>MGKVYKKVELVGTSEEGLEAAIQAALARARKTLRHLDWFEVKE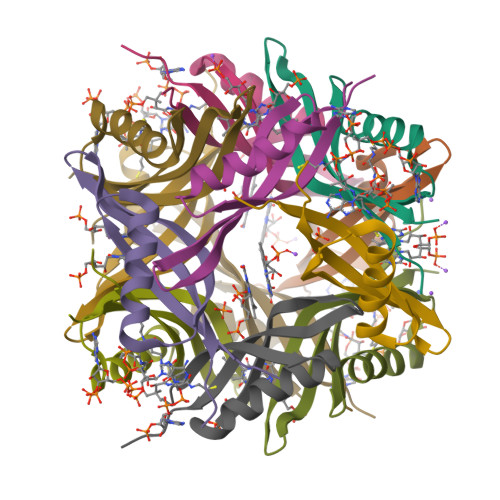IRGTIGEAGVKEYQVVLEVGFALEET[6x]2′,3′-cyclic nucleotide 3′-phosphodiesterase (CNPase) comprises 4% of total myelin protein in the central nervous system (CNS), being the most abundant CNS non-compact myelin protein4. CNPase consists of an N-terminal polynucleotide kinase-like domain10, a catalytic phosphodiesterase domain11, and a membrane-anchored C-terminal tail, which contains a cysteine residue that undergoes isoprenylation. The catalytic domain enables the rapid hydrolysis of nucleoside 2′,3′-cyclic phosphates to nucleoside 2′-phosphates. The CNPase catalytic site, lying in a groove between two lobes, has pseudo two-fold symmetry and contains two apposing His-X-Thr-X (X denotes a hydrophobic residue) motifs, characteristic for 2H phosphoesterases 113537.

We previously determined a V321A structure in complex with 2′-AMP34, in which the β5-α7 loop was open. While we have also obtained structures with an open β5-α7 loop from other mutants and the wild-type protein in complex with products, this has been particularly easy with V321A. This could relate to a higher binding affinity for the product, which would result in enzyme inhibition via hindered product release, and may explain the increased KM value. To further investigate the relevance of ligand size, we crystallized V321A in the presence of adenosine 2′,5′-bisphosphate (2′,5′-ADP), which, in addition to the 2′-phosphate, also contains a 5′-phosphate, thus mimicking the first 5′-phosphate of an RNA molecule. We obtained structures in the space groups P21 and P212121, and both structures allowed us to analyze the ligand orientation in its entirety. Similarly to V321A in complex with 2′-AMP34, the 2′,5′-ADP complexes show the β5-α7 loop the in the open conformation, with direct interactions between the 2´-phosphate and the N terminus of helix α7. The 5′-phosphate is visible and extends out of the active site towards bulk solvent. In an RNA oligonucleotide, the 5′-phosphate will be followed by another ribose and a base; several aromatic residues on the CNPase surface are in position to interact with these groups.

> GGLEKDFLPLYFGWFLTKKSSETLRKAGQVFLEELGNHKAFKKELRHFISGDEPKEKLELVSYFGKRPPGVLHCTTKFCDYGKAAGAEEYAQQEVVKRSYGKAFKLSISALFVTPKTAGAQVVLTDQELQLWPSDLDKPSASEGLPPGSRAHVTLGCAADVQPAQTGLDLLDILQQVKGGSQGEAVGELPRGKLYSLGKGRWMLSLTKKMEVKAIFTGYYG Specifically, cell death-inducing mitochondrial permeabilization is prevented by tight sequestration of membrane-localized proteins by anti-apoptotic members of the BCL-2 family, which include BCL-2, BCL-XL, BCL-W, A1, and MCL1. Consistent with its frequent amplification, MCL1 is highly expressed in many tumor types, and high expression levels of MCL1 contribute to tumor development and resistance to chemotherapy. There has been intensive effort to target anti-apoptotic members of the BCL-2 family with small molecules designed to release pro-apoptotic proteins from their sequestered state. In this report, we describe the development of a general and robust crystallography platform for soluble MCL1, using a combination of protein fusion and engineering strategies.

Using this construct, we embarked on an extensive co-crystallization screening campaign spanning structurally diverse ligands and broad matrix crystallization screens. Notably, we did not obtain crystals for apo MCL1 173–321, consistent with the apparent difficulty in obtaining a ligand-independent crystal form for MCL1. As the co-crystallization of MCL1 and ligand 1 would not be generally applicable to other ligands, we explored a protein engineering approach to develop a more robust MCL1 crystal system. As an initial proof of concept, we re-investigated the co-crystallization of ligand 1, which in earlier efforts relied entirely on zinc-mediated interactions between ligand and neighboring protein. The structure of MBP-MCL1 was determined to 2.35 Å and has high overall similarity to the structure of MCL1 173–321 (superposition r.m.s.d. of MBP-MCL1 and MCL1 173–321 bound to 1: 0.58 Å overall, calculated on all common Cα). Interestingly, in the absence of the zinc and pyrophosphate packing interactions, the pyridine ring rotates 180° from the previous non-MBP structure, with the 4-methyl group now pointing toward H224 and the imidazole group facing out towards solvent. In our own hands, removal of ligand- and zinc-mediated crystal packing revealed a new sidechain orientation where the imidazole and methyl substituents were opposite to the non-MBP structure.

> SELYRQSLEIISRYLREQATGAKDTKPMGRSGATSRKALETLRRVGDGVQRNHETAFQGMLRKLDIKNEDDVKSLSRVMIHVFSDGVTNWGRIVTLISFGAFVAKHLKTINQESCIEPLAESITDVLVRTKRDWLVKQRGWDGFVEFFHV Hydroxysteroid 17-beta-dehydrogenase 13 (HSD17B13) is a hepatic lipid droplet-associated enzyme that is upregulated in patients with non-alcoholic fatty liver disease. Recently, there have been several reports that predicted loss of function variants in HSD17B13 protect against the progression of steatosis to non-alcoholic steatohepatitis with fibrosis and hepatocellular carcinoma. Here we report crystal structures of full length HSD17B13 in complex with its NAD+ cofactor, and with lipid/detergent molecules and small molecule inhibitors from two distinct series in the ligand binding pocket. The overall structure of each HSD17B13 subunit could be divided into two parts: (i) the catalytic core domain (residues 29–259) that contained the cofactor binding site and the catalytic center and (ii) the membrane anchoring domain that consisted of the N-terminal helix (N2-P28) which was highly hydrophobic and a C-terminal proximal helix-turn-helix motif (P260-N286) which formed an amphipathic patch on the protein surface.

Subsequent mutation of four residues (G177, V178, T205, and I293) identified at the compound 1 binding site of dog HSD17B13 to the human ones (E177, G178, A205, and V293, dog mutant) further improved the resolution of these crystals (compound 1-Dog mutant). The overall structure of the compound 1 complex with dog mutant HSD17B13 did not have large changes in the catalytic cores of the HSD17B13 dimer compared to the apo HSD17B13 structure (0.31 Å for 437 Cα atoms of the dimer). Compound 1 bound to both subunits of the dog mutant HSD17B13, displacing the C-terminal peptides from the substrate sites of both subunits. Missing the anchoring to the substrate sites from the C-terminal peptides, the adjacent P274-N286 helices in the helix-turn-helix motifs became disordered. Compound 1 binding also rearranged the P218-T239 loops, which interacted with the C-terminal peptides in the apo structure. Within the loop P229-L237 peptides became disordered, and the side chain of F220 adopted a different rotamer. The combined effects of G177E and V178G mutations made an outward shift of the 177-180 peptide away from the ligand, leaving more space at the active site of the mutated dog HSD17B13 for inhibitors and substrates. As a result, 1 had full occupancies in both HSD17B13 subunits in the crystal of the mutant dog protein. Dog mutant HSD17B13 bound compound 1 strongly, and only slightly less than the human HSD17B13 (dog mutant HSD1713/compound 1 Tagg: 46.8 ± 2.2 °C; human HSD17B13/compound 1 Tagg: 49.1 ± 2.0 °C; unpaired t test p = 0.016), indicating that the mutations introduced in dog HSD17B13 based on compound 1 interactions increased its binding affinity. All of the residues interacting with 1 were from one subunit, except A205 (human sequence), which was from the second subunit of the HSD17B13 dimer.

>[2x]MGNIILDLLLLLLTIIYSYLEALVKVFFPRKRKSVAGEIVLITGAGHGIGRWTAYEFAKQKSRLVLWDINKHGVEETAAECRKLGATVHTFVVDCGNREDIYNSVKQVKKEVGDVTILVNNAGTVYPADLLSTKDEEITKTFEINILGHFWITKALLPSMIKRNHGHIVTVASVCGHEGIPYLIPYCSSKFAAVGFHRALTLELQALGITGIKTSCLCPVFVNTGFTKNPSTRLWPILETDTVARSLIDGILTNKKMIFVPSYYNIYLILDKFLPERALAAINHLQNIQFEAVVGHKTRMKGSGHHHHHHHHHHH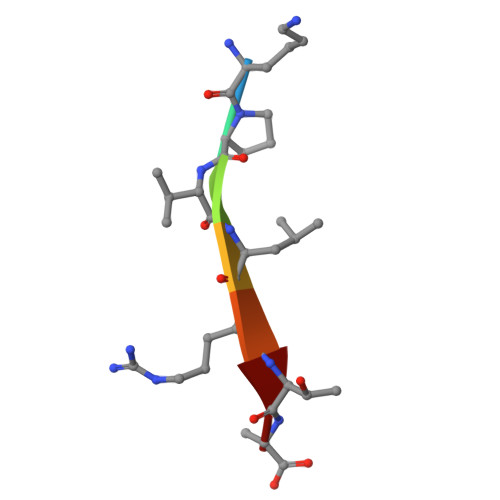> KPVLRTA> MGCDRNCGLIAGAVIGAVLAVFGGILMPVGDLLIQKTIKKQVVLEEGTIAFKNWVKTGTEVYRQFWIFDVQNPQEVMMNSSNIQVKQRGPYTYRVRFLAKENVTQDAEDNTVSFLQPNGAIFEPSLSVGTEADNF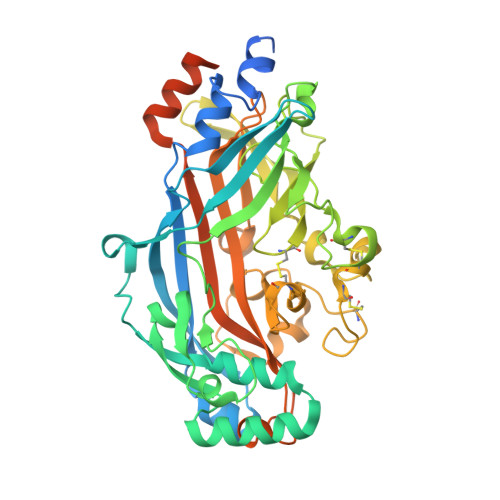TVLNLAVAAASHIYQNQFVQMILNSLINKSKSSMFQVRTLRELLWGYRDPFLSLVPYPVTTTVGLFYPYNNTADGVYKVFNGKDNISKVAIIDTYKGKRNLSYWESHCDMINGTDAASFPPFVEKSQVLQFFSSDICRSIYAVFESDVNLKGIPVYRFVLPSKAFASPVENPDNYCFCTEKIISKNCTSYGVLDISKCKEGRPVYISLPHFLYASPDVSEPIDGLNPNEEEHRTYLDIEPITGFTLQFAKRLQVNLLVKPSEKIQVLKNLKRNYIVPILWLNETGTIGDEKANMFRSQVTGKINLLGLIEMILLSVGVVMFVAFMISYCACRSKTIK> AKDIEISASESKFILEALRQNYRLDGRSFDQFRDVEITFGKEFGDVSVKMGNTKVHCRISCQIAQPYEDRPFEGLFVISTEISPMAGSQFENGNITGEDEVLCSRIIEKSVRRSGALDVEGLCIVAGSKCWAVRADVHFLDCDGGFIDASCIAVMAGLMHFKKPDITVHGEQIIVHPVNEREPVPLGILHIPICVTFSFFNPQDTEENIKGETNSEISIIDATLKEELLRDGVLTVTLNKNREVVQVSKAGGLPMDALTLMKCCHEAYSIIEKITDQILQLLKEDSEKRNKYAAMLTSENAREI;> GHMSRLEIYSPEGLRLDGRRWNELRRFESSINTHPHAADGSSYMEQGNNKIITLVKGPKEPRLKSQMDTSKALLNVSVNITKFSKFERSKSSHKNERRVLEIQTSLVRMFEKNVMLNIYPRTVIDIEIHVLEQDGGIMGSLINGITLALIDAGISMFDYISGISVGLYDTTPLLDTNSLEENAMSTVTLGVVGKSEKLSLLLVEDKIPLDRLENVLAIGIAGAHRVRDLMDEELRKHAQKRVSNASAR;> AESTTLETIEIHPITFPPEVLARISPELSLQRHLSLGIRPCLRKYEEFRDVAIENNTLSRYADAGNIDTKNNILGSNVLKSGKTIVITSITGGIIEETSASIKDLDDFGEEELFEVTKEEDIIANYASVYPVVEVERGRVGACTDEEMTISQKLHDSILHSRILPKKALKVKAGVRSANEDGTFSVLYPDELEDDTLNETNLKMKRKWSYVLYAKIVVLSRTGPVFDLCWNSLMYALQSVKLPRAFIDERASDLRMTIRTRGRSATIRETYEIICDQTKSVPLMINAKNIAFASNYGIVELDPECQLQNSDNSEEEEVDIDMDKLNTVLIADLDTEAEETSIHSTISILAAPSGNYKQLTLMGGGAKITPEMIKRSLLLSRVRADDLSTRFNI;> GHGNNKEPNTKNRLDSAEKKKKMSVQAEIGILDHVDGSSEFVSQDTKVICSVTGPIEPKARQELPTQLALEIIVRPAKGVATTREKVLEDKLRAVLTPLITRHCYPRQLCQITCQILESGEDEAEFSLRELSCCINAAFLALVDAGIALNSMCASIPIAIIKDTSDIIVDPTAEQLKISLSVHTLALEFVNGGKVVKNVLLLDSNGDFNEDQLFSLLELGEQKCQELVTNIRRIIQDNISPRLVV;> GHMSLSVAEKSYLYDSLASTPSIRPDGRLPHQFRPIEIFTDFLPSSNGSSRIIASDGSECIVSIKSKVVDHHVENELLQVDVDIAGQRDDALVVETITSLLNKVLKSGSGVDSSKLQLTKKYSFKIFVDVLVISSHSHPISLISFAIYSALNSTYLPKLISAFDDLEVEELPTFHDYDMVKLDINPPLVFILAVVGNNMLLDPAANESEVANNGLIISWSNGKITSPIRSVALNDSNVKSFKPHLLKQGLAMVEKYAPDVVRSLENL;> MNVQDRRRLLGPAAAKPMAFSNTTTHVPEKKSTDLTPKGNESEQELSLHTGFIENCNGSALVEARSLGHQTSLISAVYGPRSIRGSFTSQGTISIQLKNGLLEKYNTNELKEVSSFLMGIFNSVVNLSRYPKSGIDIFVYLTYDKDLTNNPQDDDSQSKMTSSQISSLIPHCITSITLALADAGIELVDMAGAGEANGTVVSFIKNGEEIVGFWKDDGDDEDLLECLDRCKEQYNRYRDLMISCLMNQET;> GHMSTFIFPGDSFPVDPTTPVKLGPGIYCDPNTQEIRPVNTGVLHVSAKGKSGVQTAYIDYSSKRYIPSVNDFVIGVIIGTFSDSYKVSLQNFSSSVSLSYMAFPNASKKNRPTLQVGDLVYARVCTAEKELEAEIECFDSTTGRDAGFGILEDGMIIDVNLNFARQLLFNNDFPLLKVLAAHTKFEVAIGLNGKIWVKCEELSNTLACYRTIMECCQKNDTAAFKDIAKRQFKEILTVKEE;> RSMSEVITITKRNGAFQNSSNLSYNNTGISDDENDEEDIYMHDVNSASKSESDSQIVTPGELVTDDPIWMRGHGTYFLDNMTYSSVAGTVSRVNRLLSVIPLKGRYAPETGDHVVGRIAEVGNKRWKVDIGGKQHAVLMLGSVNLPGGILRRKSESDELQMRSFLKEGDLLNAEVQSLFQDGSASLHTRSLKYGKLRNGMFCQVPSSLIVRAKNHTHNLPGNITVVLGVNGYIWLRKTSQMDLARDTPSANNSSSIKSTGPTGAVSLNPSITRLEEESSWQIYSDENDPSISNNIRQAICRYANVIKALAFCEIGITQQRIVSAYEASMVYSNVGELIEKNVMESIGSDILTAEKMRGNGN;> MKHHHHHHPMACNFQFPEIAYPGKLICPQYGTENKDGEDIIFNYVPGPGTKLIQYEHNGRTLEAITATLVGTVRCEEEKKTDQEEEREGTDQSTEEEKSVDASPNDVTRRTVKNILVSVLPGTEKGRKTNKYANNDFANNLPKEGDIVLTRVTRLSLQRANVEILAVEDKPSPIDSGIGSNGSGIVAAGGGSGAATFSVSQASSDLGETFRGIIRSQDVRSTDRDRVKVIECFKPGDIVRAQVLSLGDGTNYYLTTARNDLGVVFARAANGAGGLMYATDWQMMTSPVTGATEKRKCAKPF;> GAMSVPAIAPRRKRLADGLSVTQKVFVRSRNGGATKIVREHYLRSDIPCLSRSCTKCPQIVVPDAQNELPKFILSDSPLELSAPIGKHYVVLDTNVVLQAIDLLENPNCFFDVIVPQIVLDEVRNKSYPVYTRLRTLCRDSDDHKRFIVFHNEFSEHTFVERLPNETINDRNNRAIRKTCQWYSEHLKPYDINVVLVTNDRLNREAATKEVESNIITKSLVQYIELLPNADDIRDSIPQMDSFDKDLERDTFSDFTFPEYYSTARVMGGLKNGVLYQGNIQISEYNFLEGSVSLPRFSKPVLIVGQKNLNRAFNGDQVIVELLPQSEWKAPSSIVLDSEHFDVNDNPDIEAGDDDDNNESSSNTTVISDKQRRLLAKDAMIAQRSKKIQPTAKVVYIQRRSWRQYVGQLAPSSVDPQSSSTQNVFVILMDKCLPKVRIRTRRAAELLDKRIVISIDSWPTTHKYPLGHFVRDLGTIESAQAETEALLLEHDVEYRPFSKKVLECLPAEGHDWKAPTKLDDPEAVSKDPLLTKRKDLRDKLICSIDPPGCVDINDALHAKKLPNGNWEVGVHIADVTHFVKPGTALDAEGAARGTSVYLVDKRIDMLPMLLGTDLCSLKPYVDRFAFSVIWELDDSANIVNVNFMKSVIRSREAFSYEQAQLRIDDKTQNDELTMGMRALLKLSVKLKQKRLEAGALNLASPEVKVHMDSETSDPNE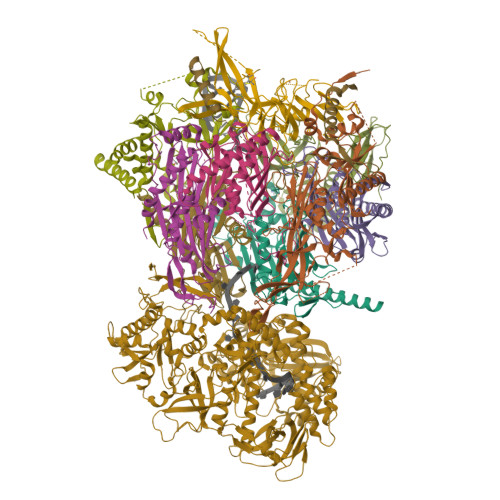VEIKKLLATNSLVEEFMLLANISVARKIYDAFPQTAMLRRHAAPPSTNFEILNEMLNTRKNMSISLESSKALADSLDRCVDPEDPYFNTLVRIMSTRCMMAAQYFYSGAYSYPDFRHYGLAVDIYTHFTSPIRRYCDVVAHRQLAGAIGYEPLSLTHRDKNKMDMICRNINRKHRNAQFAGRASIEYYVGQVMRNNESTETGYVIKVFNNGIVVLVPKFGVEGLIRLDNLTEDPNSAAFDEVEYKLTFVPTNSDKPRDVYVFDKVEVQVRSVMDPITSKRKAELLLK;> RSMEATPIPSSETKADGILLETISVPQIRDVMERFSVLCNSNISKSRAKPVTNSSILLGKILPREEHDIAYSKDGLPNKVKTEDIRIRAQNFKSALANLEDIIFEIEKPLVVPVKLEEIKTVDPASAPNHSPEIDNLDDLVVLKKKNIQKKQPAKEKGVTEKDAVDYSKIPNILSNKPG>GPGSMVQSERRRLGVMGGTFDPIHNGHLVAASEVADRFALDEVIFVPTGQPWQKQGRKVSPAEHRYLMTVIATASNPRFTVSRADIDRGGATYTVDTLTDLRTAHPDADLYFITGADALASILSWENWEQLFTLAKFIGVSRPGYELSSDHIAHAELPP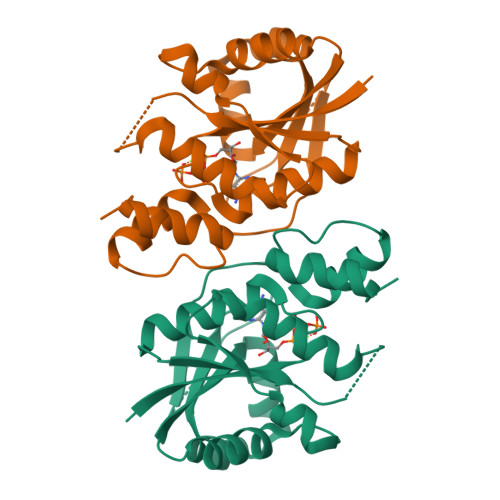DGLSLVEVPALAISSTDCRIRAGQARPIWYLVPDGVVQYVAKHRLYSGNKGNQGGLA[2x]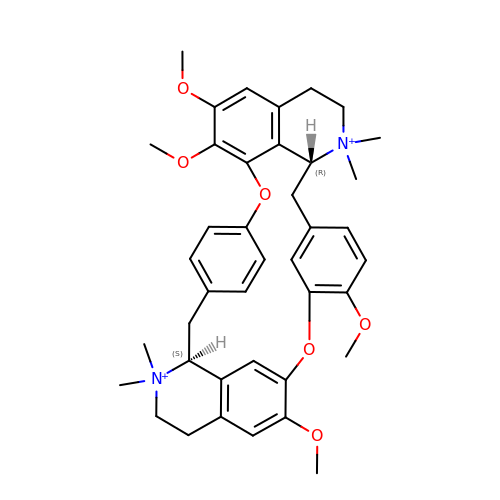6,6',7',12'-tetramethoxy-2,2,2',2'-tetramethyltubocuraran-2,2'-diium | C40 H48 N2 O6 | JFXBEKISTKFVAB-AJQTZOPKSA-N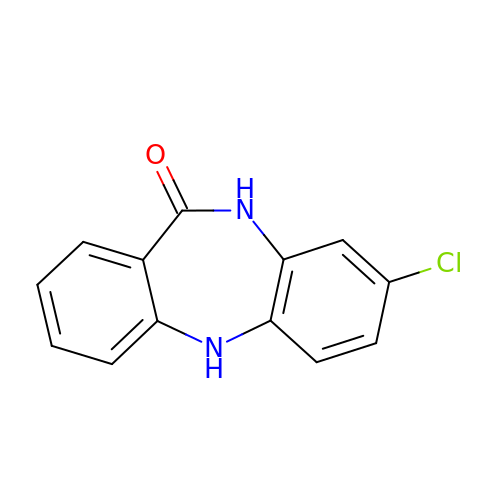8-chloro-5,10-dihydro-11H-dibenzo[b,e][1,4]diazepin-11-one | C13 H9 Cl N2 O | YVWNDABPZGGQFE-UHFFFAOYSA-N> MINIISRLQEVFGHAIKAAYPDLENPPLLVTPSQQAKFGDYQCNSAMGISQMLKTKEQKVNPREIAENITKHLPDNECIEKVEIAGPGFINVHLRKDFVSEQLTSLLVNGVQLPALGENKKVIVDFSSPNIAKEMHVGHLRSTIIGESISRLFEFAGYDVLRLNHVGDWGTQFGMLIAHLQDKFPDYLTVSPPIGDLQVFYKESKKRFDTEEEFKKRAYQCVVLLQGKNPDITKAWKLICDVSRQELNKIYDALDVSLIERGESFYQDRMNDIVKEFEDRGFVQVDDGRKIVFVPGCSIPLTIVKSDGGYTYDTSDLAAIKQRLFEEKADMIIYVVDNGQSVHFQTIFAAAQMIGWYDPKVTRVFHAGFGVVLGEDKKKFKTRSGETVRLMDLLGEGLKRSM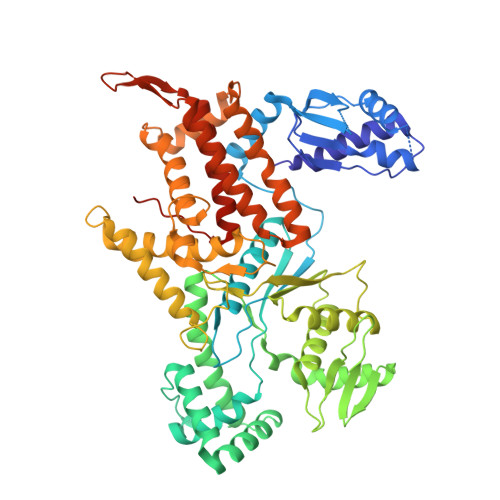DKLKEKERDKVLTAEELNAAQTSVAYGCIKYADLSHNRLNDYIFSFDKMLDDRGNTAAYLLYAFTRIRSIARLANIDEEMLQKAARETKILLDHEKEWKLGRCILRFPEILQKILDDLFLHTLCDYIYELATAFTEFYDSCYCVEKDRQTGKILKVNMWRMLLCEAVAAVMAKGFDILGIKPVQRMENLYFQSHHHHHH> MYKIKDVETRIKNDGVDLGDIGCRFYTEDENTASIRIGINDKQGRIDLKAHGLTPRLHLFMEDGSIFKNEPLIIDDVVKGFITYKIPKKVIKHAGYVRCKLFLEKEEEKIHVANFSFNIVDSGIESAVAKEIDVKLVDDAITRI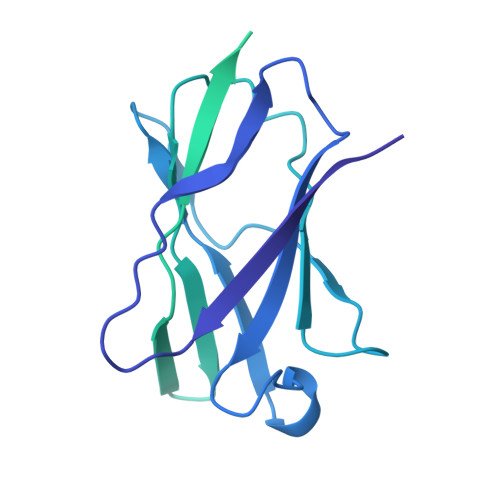LKDNATDLLSKDFKEKIDKDVISYIEKNESRFKGAKGDKGEPGQPGAKGEAGKKGEQGAPGKNGTVVSINPDTKMWQIDGKDTDIKAEPELLDKINIANVEGLEDKLQEVEKIKDTTLNDSKTYTDTKIAELVDSAPESMNTLRELAEAIQNNSISESVLQQIGSKVSTEDFEEFKQTLNDLYAPKNHNHDERYVLSSQAFTKQQADSLYQLKSASQPTVKIWTGTENEYNYIYQKDPNTLYLIKG>[3x]MALYREGKAAMAADGTVTGTGTKWQSSLSLIRPGATIMFLSSPIQMAVVNKVVSDTEIKAITTNGAVVASTDYAILLSDSLTVDGLAQDVAETLRYYQSQETVIADAVEFFKEFDFESLQNLANQIKADSEASESSAAAAAASESKAKTSEDNAKSSENAAKNSEVAAETTRDQIQQIIDNAGDQSTLVVLAQPDGFDSIGRVSSFAALRNLKPKKSGQHVLLTSYYDGWAAENKMPTGGGEFISSIGTATDDGGYIAAGPGYYWTRVVNNNSFTAEDFGCKTTATPPPNFNVLPAELFDNTARMQAAFNLAISKSFKLNLSAGTYYFESSDTLRITGPIHIEGRPGTVFYHNPSNKANPKTDAFMNISGCSMGRISSINCFSNSYLGKGINFDRSVGDNRKLVLEHVYVDTFRWGFYVGEPECINQIEFHSCRAQSNYFQGIFIESFKEGQEYGHSAPVHFFNTICNGNGPTSFALGATYKTTKNEYIKVMDSVNDVGCQAYFQGLSNVQYIGGQLSGHGSPRNTSLATITQCNSFIIYGTDLEDINGFTTDGTAITADNIDTIESNYLKDISGAAIVVSSCLGFKIDSPHIFKIKTLSTIKLMNNTYNYEIGGFTPDEALKYNVWDANGLATNRISGVIHPRLVNSRLGINSVAFDNMSNKLDVSSLIHNETSQIIGLTPSTGSNVPHTRIMWSNGAMYSSTDLNNGFRLNYLSNHNEPLTPMHLYNEFSVSEFGGSVTESNALDEIKYIFIQTTYANSGDGRFIIQALDASGSVLSSNWYSPQSFNSTFPISGFVRFDVPTGAKKIRYGFVNSANYTGSLRSHFMSGFAYNKRFFLKIYAVYNDLGRYGQFEPPYSVAIDRFRVGDNTTQMPSIPASSATDVAGVNEVINSLLASLKANGFMSS

In the present study, Klebsiella phage GH-K3-derived depolymerase Depo32 (encoded by gene gp32) was identified to exhibit high efficiency in specifically degrading the CPSs of K2 serotype K. pneumoniae. Phage depolymerases specifically recognize the glycosidic bonds on the host surface and randomly degrade them to release the repeating units (oligosaccharides) of the glycopolymers; thus, the phage particles can move closer to the cell surface and bind to host receptors. Here, GH-K3 gp32 was identified to encode a depolymerase, Depo32, which efficiently degrades the CPSs of K. pneumoniae K7 (K2 capsular type). In summary, Depo32 effectively binds and cleaves the CPSs of K2 capsular type K. pneumoniae via the putative active center constituted by Glu545/Glu423 and Asp546/Glu423 and initiates the hydrolysis process, causing the pathogens to become sensitive to elimination by the host immune system and thus achieving protective effects.

To understand the whole architecture as well as the potential modes of action of Depo32 on the K2-type CPS of K. pneumoniae, the structure of Depo32 was solved by cryo-electron microscopy (cryo-EM). Atomic models were built into the 2.46 Å nonsymmetrized and 2.32 Å C3-symmetrized maps and refined iteratively in real and reciprocal spaces. Both the nonsymmetrized and C3-symmetrized maps presented well-defined electron densities in the core region, and they all revealed trimeric architectures, similar to the overall characteristics of the previously identified tailspike proteins with known structures (Fig. 2A through C). In the core region of Depo32, since the resolution of the C3-symmetrized map is slightly higher than that of the nonsymmetrized map, and because of the inclusion of the potential CPS binding, catalytic and/or regulatory domains in this region, we then focused on the C3-symmetrized map and model to perform the subsequent analyses. In addition to the invisible N-terminal anchor domain and the helical-bundle domain (to residue 185) that may form the head of the spike protein, the remaining core region of the Depo32 monomer can be further split into the following domains: (i) a very short neck helix and the connection domain (residues 186–271), (ii) the β-helix domain (residues 272–642), (iii) the connection helix domain (residues 643–666), (iv) the carbohydrate-binding module (CBM) (residues 667–846), and (v) a C-terminal domain (residues 847–907). The three β-helix domains from the Depo32 trimer form a left-handed coiled β-coil architecture that is mainly mediated by polar interactions, whereas the residues inside the β-helical solenoid are highly hydrophobic. Through comprehensive inspection of the single β-helix domain or the trimer of Depo32, it was observed that both the intra- and intermolecular surface pockets were flanked by pairs of Asp/Glu residues, and the substrate oligosaccharides might associate at this location and be cleaved.>MIQQTGYSKKVMEHFMNPRNVGVIDDPDGYGKVGNPVCGALMEIFIKVGDEKIEDIKFRTFGCGAAIATSSMITEMARGKSLEEAMRITRNDVADALDGLPPQKMACSNLAADALHAA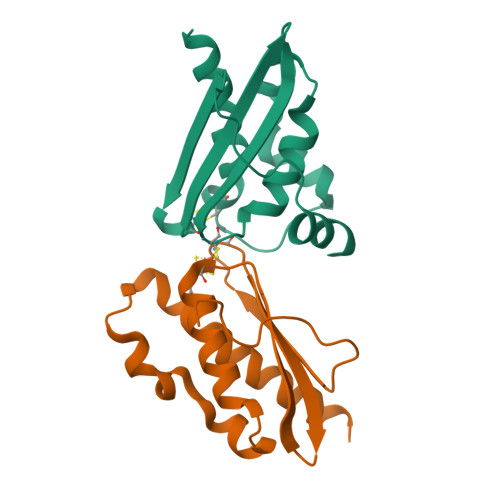INDYLSKKQKHLEHHHHHH[4x]>[4x]GKAFDDGAFTGIREINLSYNKETAIGDFQVVYDLNGSPYVGENHKSFITGFTPVK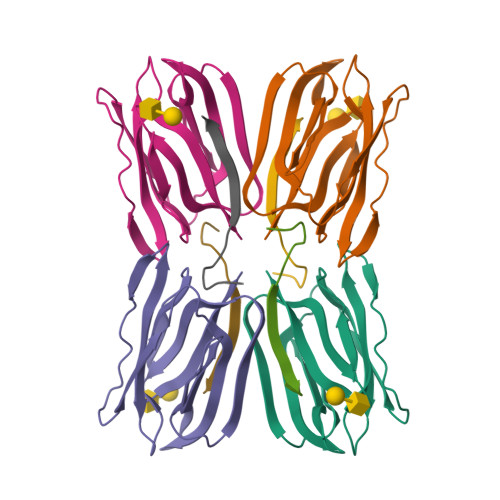ISLDFPSEYIMEVSGYTGKVSGYVVVRSLTFKTNKKTYGPYGVTSGTPFSLPIENGLIVGFKGSIGYWLDYFSMYLSL;>NEQSGISQTVIVGPWGAQVST[4x]> QQQQCRQQFQTQQRLRACQRVIRRWSQGGGPMEDVEDEIDETDEIEEVVEPDQAARPPTLQRCCQQLRNISPQCRCPSLRQAVQSAQ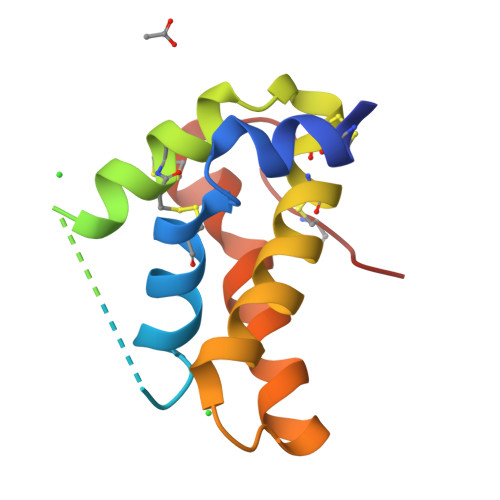QQQGQVGPQQVGHMYRVASRIPAICNLRPMSCPFRQQ>MYYPFVRKALFQLDPERAHEFTFQQLRRITGTPFEALVRQKVPAKPVNCMGLTFKNPLGLAAGLDKDGECIDALGAMGFGSIEIGTVTPRPQPGNDKPRLFRLVDAEGLINRMGFNNLGVDNLVENVKKAHYDGVLGINIGKNKDTPVEQGKDDYLICMEKIYAYAGYIAINISSP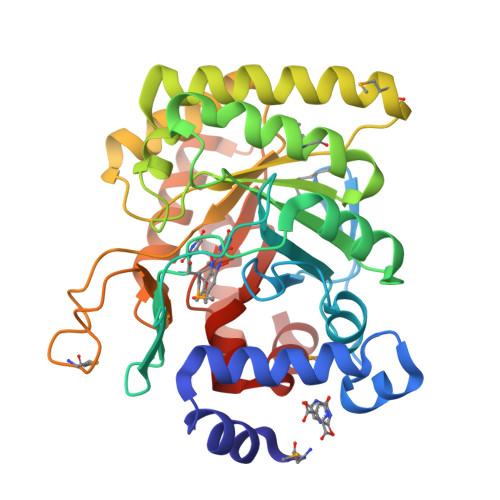NTPGLRTLQYGEALDDLLTAIKNKQNDLQAMHHKYVPIAVKIAPDLSEEELIQVADSLVRHNIDGVIATNTTLDRSLVQGMKNCDQTGGLSGRPLQLKSTEIIRRLSLELNGRLPIIGVGGIDSVIAAREKIAAGASLVQIYSGFIFKGPPLIKEIVTHI[4x]4-cyclohexylbenzoic 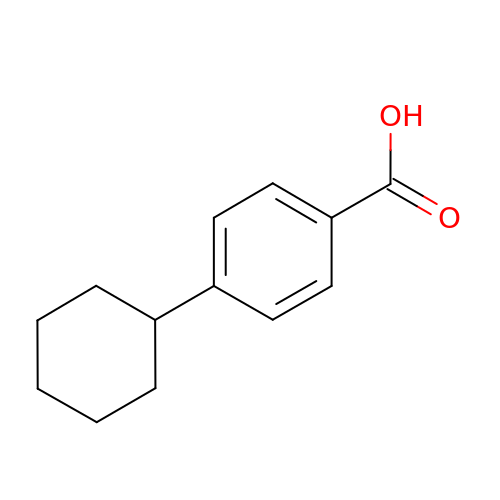acid | C13 H16 O2 | QCIWHVKGVVQHIY-UHFFFAOYSA-N> MTRDQNGTWEMESNENFEGYMKALDIDFATRKIAVRLTQTKVIDQDGDNFKTKTTSTFRNYDVDFTVGVEFDEYTKSLDNRHVKALVTWEGDVLVCVQKGEKENRGWKQWIEGDKLYLELTCGDQVCRQVFKKKLVPR

Present in the small intestine, cellular retinol binding protein 2 (CRBP2) plays an important role in the uptake, transport, and metabolism of dietary retinoids. All CRBPs share the same protein structure architecture. These small soluble proteins fold into a single β-barrel that shields the central hydrophobic cavity that constitutes a solitary binding site for retinoids. Access to the binding pocket is governed by a “portal region” composed of conformationally flexible loops connecting neighboring β-strands. By examining chemical libraries of bioactive lipids, we provided evidence for the selective interaction of CRBP2 with a subset of nonretinoid ligands with the highest affinity for sn-1 and sn-2 MAGs that contain polyunsaturated C18-C20 acyl chains.

A similar Kd was measured for 2-palmitoyl glycerol (2-PG; Kd = 51.2 ± 7.7 nM). However, how can the relatively good binding of 2-PG and 2-LaG be explained if their 16- and 12-carbon acyl chains are too short to interact with the β3-β4 loop? The answer to this question can be determined from the structures of CRBP2 complex in these lipids. They revealed an unexpected change in the orientation of the palmitoyl and lauroyl chains as compared with longer acyl moieties. In contrast, the palmitoyl in 2-PG adapted an inverse orientation, twisting first toward the β3-β4 loop before interacting with the α-helices II and I. Thus, the interaction with the β3-β4 loop is prioritized, enabling the stabilization of the ligand inside the binding cavity and the protein as whole in the holoconfiguration. The presence of two alternative binding modes that depend on the length of the acyl chains explains the significant decline in the affinity of MAGs with fatty acid moieties shorter than 16 carbon atoms. The inability to stabilize the close conformation most likely contributes to the rapid diffusion of the ligand out of the binding pocket. This hypothesis is further supported by the comparison of normalized crystallographic B-factors calculated for CRBP2 in complex with 2-AG or 2-OG and 2-PG or 2-LaG. The binding of MAGs with shorter and saturated fatty acid chains results in a significant increase in the structural dynamics of α-helix I and β3-β4 loop of the protein's entry port.>MVPAQHRPPDRPGDPAHDPGRGRRLGIDVGAARIGVACSDPDAILATPVETVRRDRSGKHLRRLAALAAELEAVEVIVGLPRTLADRIGRSAQDAIELAEALARRVSPTPVRLADERLTTVSAQRSLRQAGVRASEQRAVIDQAAAVAILQSWLDERLAAMA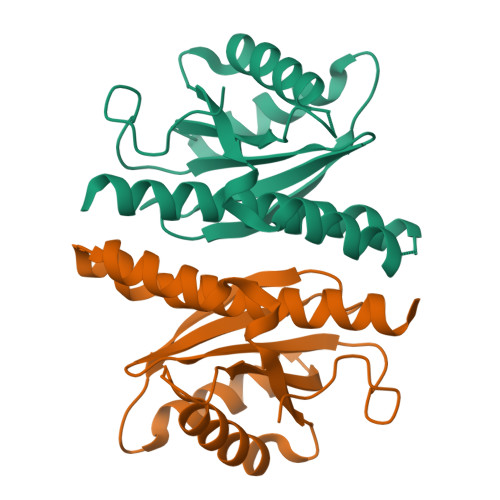GTQEGSDA[2x]>ISHMIQNRAQAVDQLRAVARYFRQTEPHSPVAYLADKAAEWADMPLHKWLESVVKDDGSLSHIRELLGVRPD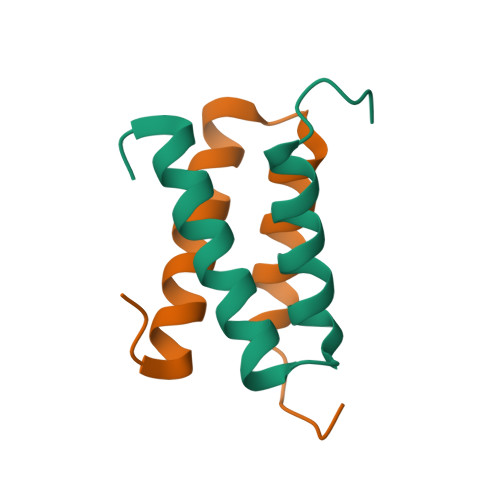EQS[2x]>[4x]MSELEKAVVALIDV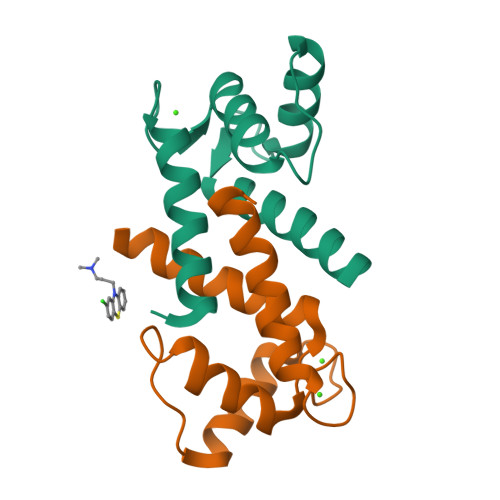FHQYSGREGDKHKLKKSELKELINNELSHFLEEIKEQEVVDKVMETLDSDGDGECDFQEFMAFVAMITTACHEFFE>[2x]MNMVMLTIDGKQVQVEKGTTIKKAAEKLGIEIPGLCDDNDLKPFGACRLCVVEDARGNLVASCHTPVREGMVVKTNSPKVLKARRVILELLLSSHNADCFECDKNLHCKLQKYAYELNIRNIRFKGEKRNYEIKDNGPIYYDPNKCILCGKCVRICEEVQHICAIDFASRGFKAYISTPFEKPLLESDCIFCGQCVRVCPTGALAEKTDIERIYEAISDPNKVVVVQVAPAVRVALGEEFGLEPGEIVTGKMVAALKRLGFDKVFDTQFAADMTIVEETAELVERLEKGENFPMFTSCCPSWILAVEKFYPELIPNISTARSPQQIFGAIAKNYYAKKIGVARENMFVVSVMPCIGKKFEATRPEFNNDVDAVLTTRELARMIKESGIDFIKLEEENFDSPLGESTGAAAIFGVTGGVMEAALRTAYSIMTGEELEGDKIEFTAVRGLEGIKEAEVDIKGKKVRIAIANGIGNAKKLIEKIKSGETKYDFVEVMACPGGCMSGGGQPYTDDPEFRKKRMEGIYKNDRNLPKRKSHENEEVKKVYEEYYEKPCGPKAHEELHTHYHSRKKEY;>MVKLKSIQELENLREKIKEAKKKEKIVIRICGGTGCRASGSLAVRDELVKVLKREGFANVDVNLSSDCLENTSEVHVKMTGCQGFCAQGPLMTIEPLGVFYVGVKPEDVEEIVEKSIKKNEIIERLLYHDPATGKTYVKRDENPFYAKQTRLVLKHCGTVDPASVYDYIAEGGYSAIAKALT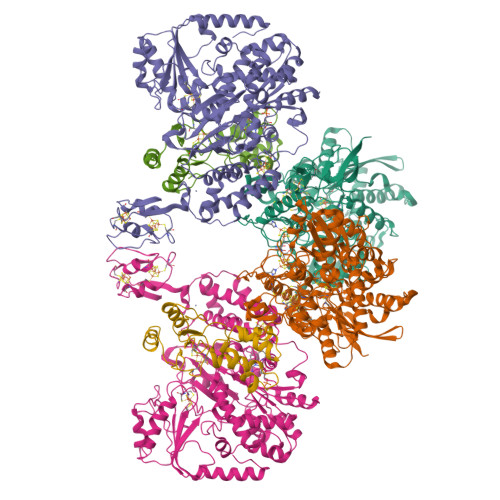MDRKQIIDEVIKSGLRGRGGAGFPTGEKWLGAYKNQSPKKYIICNGDEGDPGAFMDRSVMEGDPHKVIEGMMIGAYAIGSDEGYIYVRAEYPLAVQMLRKAIEECEKLGLLGDNILGTGFSFRLHVREGAGAFVCGESTALTYSIEGKRGMPRVRPPRTNECGLWEMPTVLNNVETFACIPEIILNGGEWFASIGTPTSTGTKIFALSGKVNRTGLVEVPMGLKLRELIFDIGGGIANNKKFKAVQLGGPSGGCVPESQLDLPIDFDSLSKAGAIMGSGGVVVVDEDTCMVDFAKFFTNFIVEESCGKCIPCREGNKKMLEILERITEGKGKEGDIELLEELGDVIISASLCGLGKTAPNPVLSTIKHFRDEYEAHIRDKKCPAGACQALAAYKIDPGKCIGCGKCVKVCPVGAISGEKKKPHVIDQSKCIKCGACAENCPKGAIYKG[2x];>MCNCCCKGSKDPRFEKVDEILSKLANERGALIAILQHVQHEFGYLPEDVIFYIASKTGIPASKIYGVATFYAQFHLKPRGKYVIRVCLGTACHVKGANKILAEFEKQLGIKAGETTSDLKFTLERVGCLGACGLAPTVMVNEKTYGKMTPEKVSEVLKEYSDVEAAASAQ[2x]>[2x]AYTTFSQTKNDQLKEPMFFGQPVNVARYDQQKYDIFEKLIEKQLSFFWRPEEVDVSRDRIDYQALPEHEKHIFISNLKYQTLLESIQGRSPNVALLPLISIPELETWVETWAFSETIHSRSYTHIIRNIVNDPSVVFDDIVTNEQIQKRAEGISSYYDELIEMTSYWHLLGEGTHTVNGKTVTVSLRELKKKLYLCLMSVNALEAIRFYVSFACSFAFAERELMEGNAKIIRLIARDEALHLT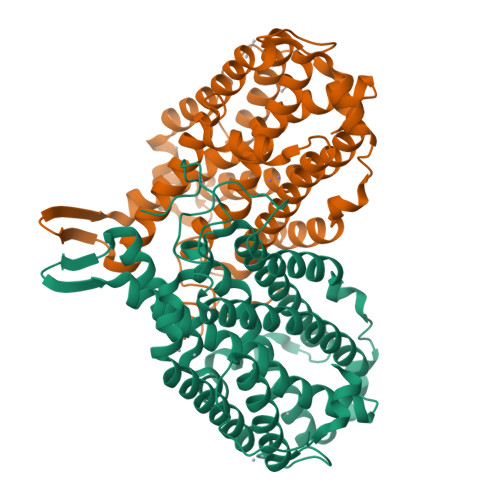GTQHMLNLLRSGADDPEMAEIAEECKQECYDLFVQAAQQEKDWADYLFRDGSMIGLNKDILCQYVEYITNIRMQAVGLDLPFNTRSNPIPWINTWL> XXXXXXXXXXXXXXVNLAEVERLARSADAPRGFANALL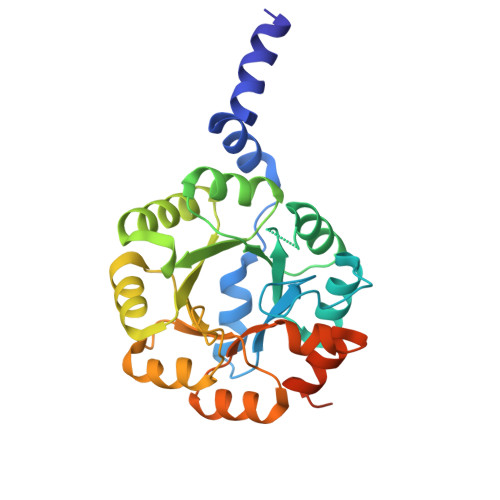ERAKRKEPAVIAEIKKASPSKGVLREHFVPAEIARSYEAGGAACLSVLTDVDFFQGADAYLKEARAACALPVIRKDFMIDPYQIVEARAIGADCILLIVSALDDVLMAELAATAKSVGLDVLVEVHDGTELERALKTLDTPLVGINNRNLHTFEVSLETTLDLLPEIPRDRLVVTESGILNRADVELMEVSEVYAFLVGEAFMRADDPGLELKRLFFQERGAVVLGADPDTSGHHHHHH Spliceostatin E (form I) | C26 H37 N 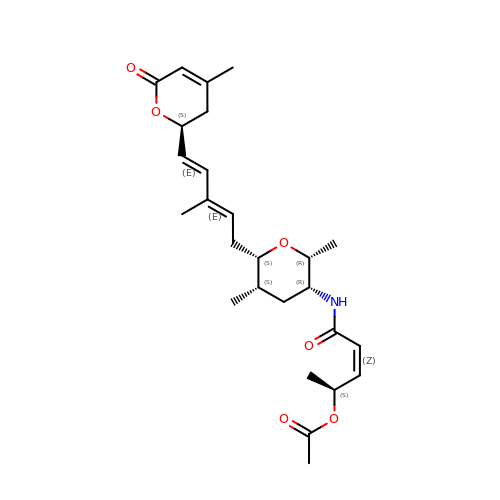O6 | CDYGVGCTHMNLJY-FLMQFJOVSA-N> GSPSRSVKLAGNSSLCPVSGWAIYSKDNSVRIGSKGDVFVIREPFISCSPLECRT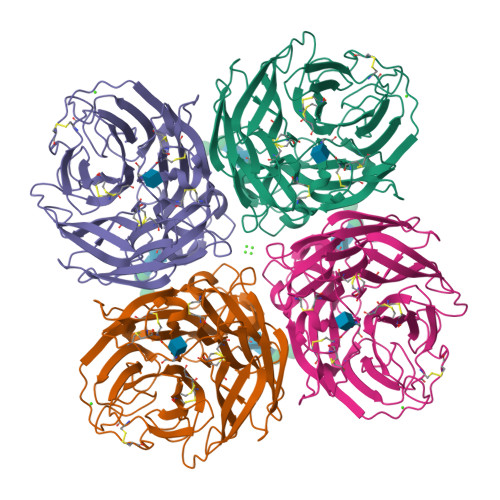FFLTQGALLNDKHSNGTIKDRSPYRTLMSCPIGEVPSPYNSRFESVAWSASACHDGINWLTIGISGPDSGAVAVLKYNGIITDTIKSWRNNILRTQESECACVNGSCFTIMTDGPSDGQASYKIFRIEKGKIIKSVEMKAPNYHYEECSCYPDSSEITCVCRDNWHGSNRPWVSFNQNLEYQMGYICSGVFGDNPRPNDKTGSCGPVSSNGANGVKGFSFKYGNGVWIGRTKSISSRKGFEMIWDPNGWTGTDNKFSIKQDIVGINEWSGYSGSFVQHPELTGLDCIRPCFWVELIRGRPEENTIWTSGSSISFCGVNSDTVGWSWPDGAELPFTIDK> AKEAPQAHKAVELSILHINDHHSYLEPHETRINLNGQQTKVDIGGFSAVNAKLNKL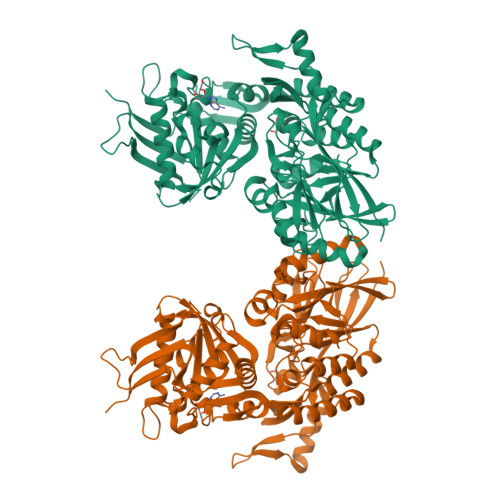RKKYKNPLVLHAGDAITGTLYFTLFGGSADAAVMNAGNFHYFTLGNHEFDAGNEGLLKLLEPLKIPVLSANVIPDKSSILYNKWKPYDIFTVDGEKIAIIGLDTVNKTVNSSSPGKDVKFYDEIATAQIMANALKQQGINKIILLSHAGSEKNIEIAQKVNDIDVIVTGDSHYLYGNDELRSLKLPVIYEYPLEFKNPNGEPVFVMEGWAYSAVVGDLGVKFSPEGIASITRKIPHVLMSSHKLQVKNSEGKWAELTGDERKKALDTLKSMKSISLDDHDAKTDKLIAKYKSEKDRLAQEIVGVITGSAMPGGSANRIPNKAGSNPEGSIATRFIAETMYNELKTVDLTIQNAGGVRADILPGNVTFNDAYTFLPFGNTLYTYKMEGSLVKQVLEDAMQFALVDGSTGAFPYGAGIRYEANETPNAEGKRLVSVEVLNKQTQQWEPIDDNKRYLVGTNAYVAGGKDGYKTFGKLFNDPKYEGVDTYLPDAESFIKFMKKHPHFEAYTSSNVKFNASTDALPKK>[2x]GAASEAEYGKVSKAWTLHADGSQEYRSSMELTLFTHTAM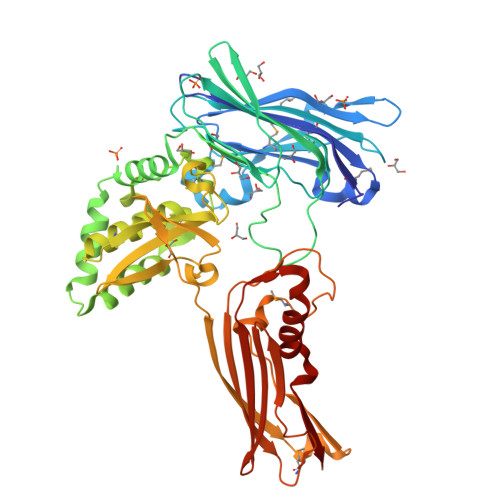NSTYGESFIVYNPDFQTLKIHSSYTRQKDGTIVKTPDNAFVEVLPRFAADAPAYNQLKEMVVVHTGLELGATIYLDYSIITKPGYYPALDINERLQETSPVKECKVSISVPEGTPLACGLYGSPVKAVEESHDGIKEVHWTLRNIPASSREAFQPKNREASPHLVASTYPSGKAALATLDKRLKESQGYESKTFAQFLTDKSGNEQEKVNIIRDHILNNLSTCPIPMAMTGYTVRDIDTVLRSAYGTPLEIAQLLNVMLNAAGIPSEVLAVYPGHLDTDACGLAAIQTLAVKATVDGKDQYLSASPLTNRGGLDKVVSLSGTSIEIETTPIQIKESRSVAISADQAKDGFAICVLPAISAGIDSWGMSALNSKRSNLFELPSLIREEVTYTVTPAEGMKLQTSTQEQVISKPFGKVTRTITPRGNTIEVVRTIELNKQQFTPAEYSDVRSLIHEWTNPDNRVLLFSL> SNAMAESLITKKAIAGGLMELCQHKRFEKIS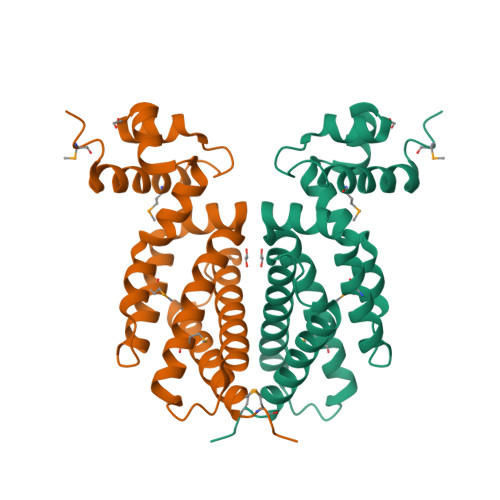IADITNICGLNRQTFYYHFTDKYDLLTWTYENDFFHCLADGITLGNWDKHVLKMLESIKENADFYKNTVSADASILSFCFSKLTNSLFMDLFEKIDTNATVNEADRVFYAEFFSYGCSGVLIKWITRGFKEAPETIANQLFRLAKDTEFLANSMYREN>[4x]MATVQPIVNSHLSELDEDVFHHFGFTTKSFDFKEKFGDVKFVCVCGSSGRIHNFAISMAKLAGLALPVENIAGSHARFVLYKVDHILFADHGMGIPSALIMLHEVTKLLHYAGCKDVLFIRLGTSGGLGVKPGTIVLSDRCVNTKLEPYNELCILGKPVRRQTIVDLNTVNELKKLSENLSLECSVVVGGTIAANDFYEEQGRLDGSICTFSKEEKLAFLQSAYEHGIRNMEME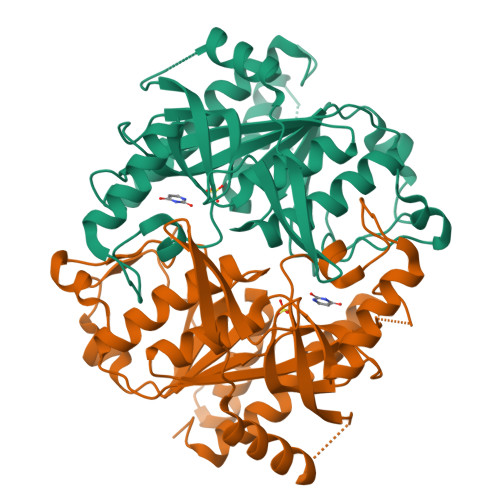GTAITSHCYLTGHRAILVCVTAVNRLEGDQITISTDEFTLFAQRPGQLVGEYLKRNNGIIVR> MAVNPELAPFTLSRGIPSFDDQALSTIIQLQDCIQQAIQQLNYSTAEFLAELLYAECSILDKSSVYWSDAVYLYALSLFLNKSYHTAFQISKEFKEYHLGIAYIFGRCALQLSQGVNEAILTLLSIINVFSSNSSNTRINMVLNSNLVHIPDLATLNCLLGNLYMKLDHSKEGAFYHSEALAINPYLWESYEAICKMRATVDLKRVFFDIAGKKSNSHNNNAASSFPSTSLSHFEPRSQPSLYSKTNKNGNNNINNNVNTLFQSSNSPPSTSASSFSSIQHFSRSQQQQANTSIRTCQNKNTQTPKNPAINSKTSSALPNNISMNLVSPSSKQPTISSLAKVYNRNKLLTTPPSKLLNNDRNHQNNNNNNNNNNNNNNNNNNNNNNNNIINKTTFKTPRNLYSSTGRLTTSKKNPRSLIISNSILTSDYSITLPEIMYNFALILRSSSQYNSFKAIRLFESQIPSHIKDTMPWCLVQLGKLHFEIINYDMSLKYFNRLKDLQPARVKDMEIFSTLLWHLHDKVKSSNLANGLMDTMPNKPETWCCIGNLLSLQKDHDAAIKAFEKATQLDPNFAYAYTLQGHEHSSNDSSDSAKTCYRKALACDPQHYNAYYGLGTSAMKL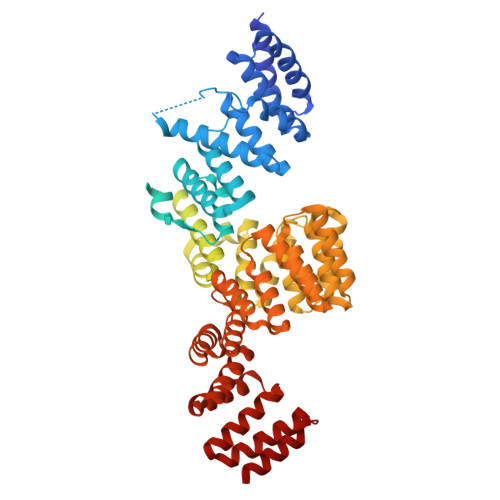GQYEEALLYFEKARSINPVNVVLICCCGGSLEKLGYKEKALQYYELACHLQPTSSLSKYKMGQLLYSMTRYNVALQTFEELVKLVPDDATAHYLLGQTYRIVGRKKDAIKELTVAMNLDPKGNQVIIDELQKCHMQE>MRIEAAELRILELPLKFRFETSFGVQTKRTILLLRLFGEGLEGLGE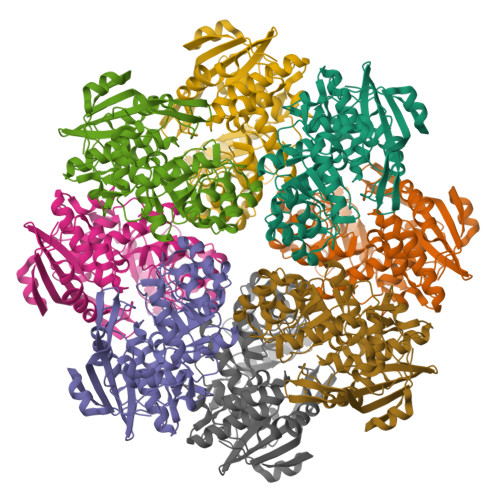GVMERLPLYREETVAGARYLLEEVFLPRVLGRDLPNPEALREALAPFRGNPMAKAVLEMAFFDLWAKALGRPLWQVLGGVRQAVEVGVSLGIQPSVEDTLRVVERHLEEGYRRIKLKIKPGWDYEVLKAVREAFPEATLTADANSAYSLANLAQLKRLDELRLDYIEQPLAYDDLLDHAKLQRELSTPICLDESLTGAEKARKAIELGAGRVFNVKPARLGGHGESLRVHALAESAGIPLWMGGMLEAGVGRAHNLHLATLPGFTKPGDVSSASRYWEEDIVEEALEAKDGLMPVPEGVGIGVHLKLPFVERVTLWQRYMSAS[2x]>[2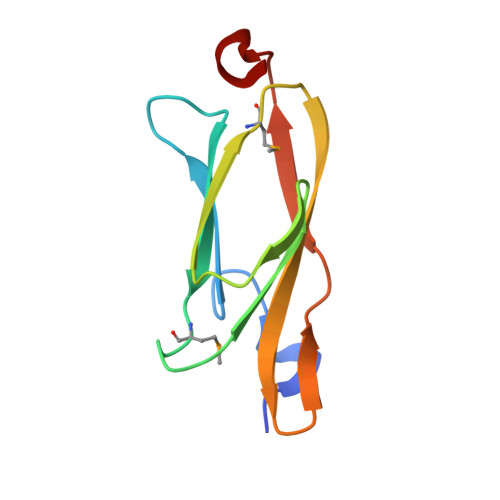x]SNAVTVDDLVEGIAFSITHDSENPNIVYLKSLMPSSYQVCWQHPQGRSQEREVTLQMPFEGKYEVTFGVQTRGGIVYGNPATFTIDSFCADFVN>MPYVEIIEQPKQRGMRFRYKCEGRSAGSIPGERSTDTTKTHPTIKINGYTGPGTVRISLVTKDPPHRPHPHELVGKDCRDGYYEAEFGPERRPLFFQNLGIRCVKKKEVKEAIILRISAGINPFNVPEQQLLDIEDCDLNVVRLCFQVFLPDEHGNFTTALPPIVSNPIYDNRAPNTAELKICRVNRNSGSCLGGDEIFLLCDKVQKEDIEVYFTGPGWEARGSFSQADVHRQVAIVFRTPPYADP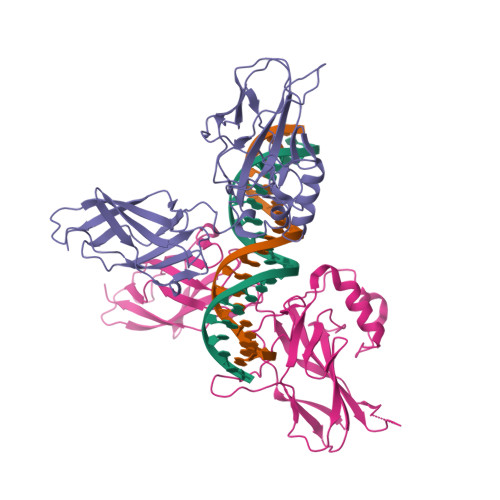SLQAPVRVSMQLRRPSDRELSEPMEFQYLPD[8x]>MSVIKPDMKIKLRMEGAVNGHPFAIEGVGLGKPFEGKQSMDLKVKEGGPLPFAYDILTTVFCYGNRVFAKYPENIVDYFKQSFPEGYSWERSMNYEDGGICNATNDITLDGDCYIYEIRFDGVNFPANGPVMQKRTVKWEPSTEKLYVRDGVLKGDVNMALSLEGGGHYRCDFKTTYKAKKVVQL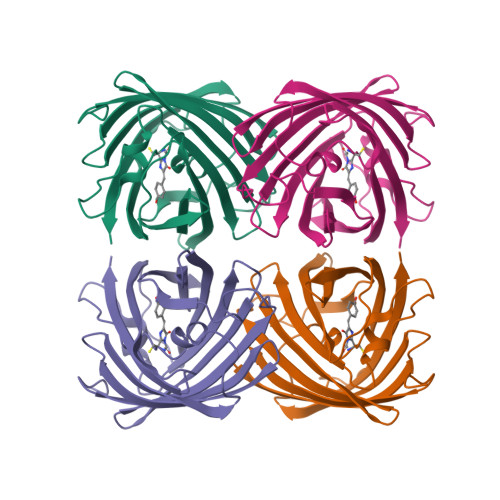PDYHFVDHHIEIKSHDKDYSNVNLHEHAEAHSELPRQAK[6x]DODECANE-TRIMETHYLAMINE 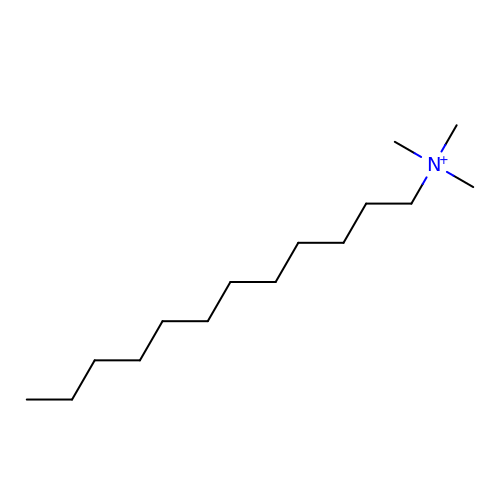| C15 H34 N | VICYBMUVWHJEFT-UHFFFAOYSA-N(2S)-3-(3-{[4-(2-aminoethoxy)-2',6-dimethyl[1,1'-biphenyl]-3-yl]amino}-1H-pyrazol-1-yl)-2-methoxypropan-1-ol 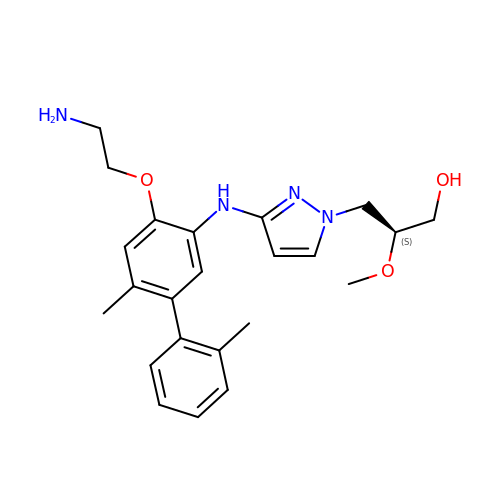| C23 H30 N4 O3 | PUPHJJGGIHFEJD-SFHVURJKSA-N N-{[(1R,2R,3R,7S,7aR)-1,2,7-trihydroxyhexahydro-1H-pyrrolizin-3-yl]methyl}acetamide 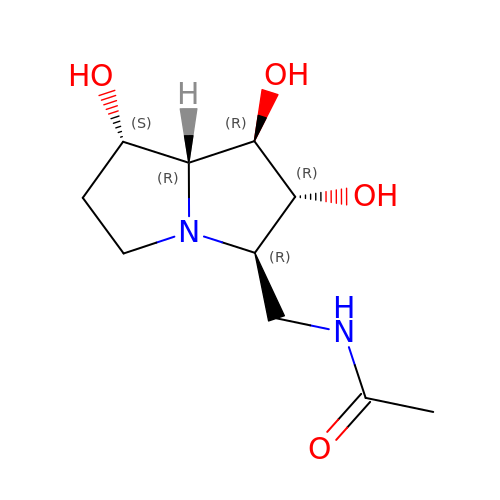| C10 H18 N2 O4 | HSDCYPQIPOCAJF-JDDHQFAOSA-N3-BUTYLTHIOLANE 1-OXIDE | C8 H16 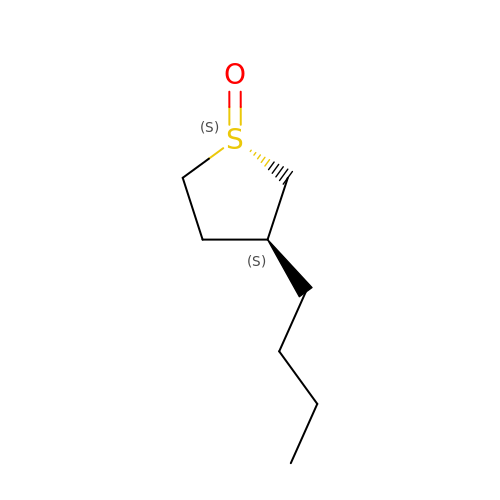O S | QVVQIIIFHZDBDL-WPRPVWTQSA-N> HHHHATIKQRTLKNIIRATGVGLHSGEKVYLTLKPAPVDTGIVFCRTDLDPVVEIPARAENVGETTMSTTLVKGDVKVDTVEHLLSAMAGLGIDNAYVELSASEVPIMDGSAGPFVFLIQSA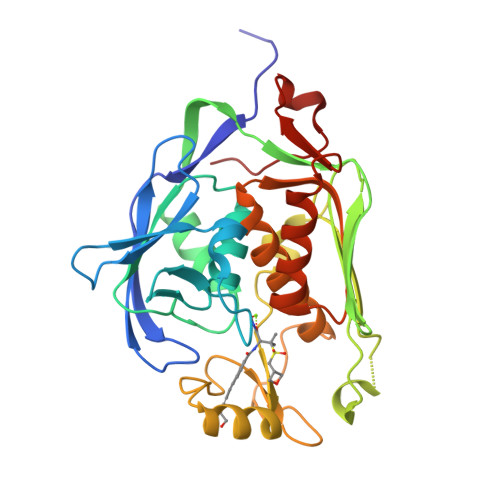GLQEQEAAKKFVRIKREVSVEEGDKRAVFVPFDGFKVSFEIDFDHPVFRGRTQQASVDFSSTSFVKEVSRARTFGFMRDIEYLRSQNLALGGSVENAIVVDENRVLNEDGLRYEDEFVKHKILDAIGDLYLLGNSLIGEFRGFKSGHALNNQLLRTLIADKDAWEVVTFEDARTAPISYMRP> GNPIHDRTSDYHKYLKVKQGDSDLFKLTVSDKRYIWYNPDPKERDSYECGEIVSETSDSFTFKTVDGQDRQVKKDDANQRNPIKFDGVEDMSEL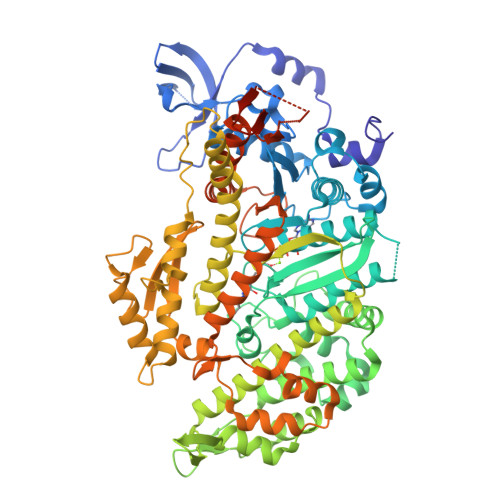SYLNEPAVFHNLRVRYNQDLIYTYSGLFLVAVNPFKRIPIYTQEMVDIFKGRRRNEVAPHIFAISDVAYRSMLDDRQNQSLLITGESGAGKTENTKKVIQYLASVAGRNQANGSGVLEQQILQANPILEAFGNAKTTRNNNSSRFGKFIEIQFNSAGFISGASIQSYLLEKSRVVFQSETERNYHIFYQLLAGATAEEKKALHLAGPESFNYLNQSGCVDIKGVSDSEEFKITRQAMDIVGFSQEEQMSIFKIIAGILHLGNIKFEKGAGEGAVLKDKTALNAASTVFGVNPSVLEKALMEPRILAGRDLVAQHLNVEKSSSSRDALVKALYGRLFLWLVKKINNVLCQERKAYFIGVLDISGFEIFKVNSFEQLCINYTNEKLQQFFNHHMFKLEQEEYLKEKINWTFIDFGLDSQATIDLIDGRQPPGILALLDEQSVFPNATDNTLITKLHSHFSKKNAKYEEPRFSKTEFGVTHYAGQVMYEIQDWLEKNKDPLQQDLELCFKDSSDNVVTKLFNDPNIASRAKKGANFITVAAQYKEQLASLMATLETTNPHFVRCIIPNNKQLPAKLEDKVVLDQLRCNGVLEGIRITRKGFPNRIIYADFVKRYYLLAPNVPRDAEDSQKATDAVLKHLNIDPEQYRFGITKIFFRAGQLARIEEARELPN SKI-O-592 | C25 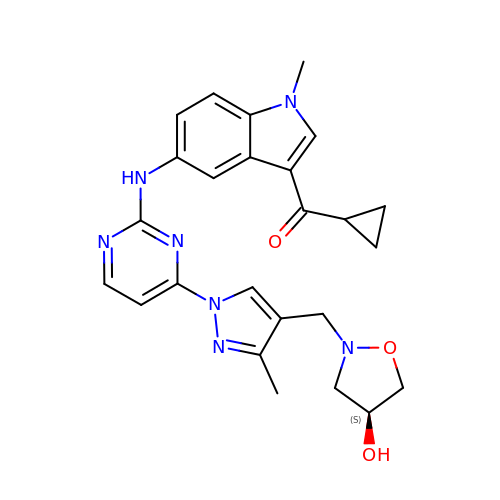H27 N7 O3 | YCZUBLQESBVOSH-IBGZPJMESA-N>MDGGMWLMQQINGQVARMKSLGMQLEAADIYNPNGSSLKDAVVMFDGGCTGVLVSNQGLLLTNHHCGYDQIQKHSSVQHNYLKDGFWSYSLAEELVNPGLEVEIVDEITDVTAAVKKELERIKKPSGLEFLSPRYLSSLAPEIVGKKAASRPGYRYEIKAFYGGNRYYMFTKKVFRDVRLVAAPPSSIGKFGSDTDNWAWPRHTGDFSIFRLYADKNGNPAEYSKDNVPYRPKRWVKVNAQGVKEGDFALIMGYPGTTYKFFTADEVTEWSEIDNNIRIEMRGILQDVMLREMLADPKINIMYAAKYASSQNGYKRAQGANWAIRRRSLREIKLAQQQEVLAWAKQKGIATTEEAVRAISKAIEGRQDLRMRQRYLLEGILMGIEMSNAPAADSDIADHWDDPARREAGLQSIRKQFEAFFNKDYSPEVEKDQLAIALLTRYAERIPAEKQPISIREGIAEYGSAKAYVEMIFDKSIYASRERFEEFMKNPDRDRLLRDPMSRFAASVAYEHQKLAKEVAAFDAPLAAAQRSYVASVLDMKGQPNLAPDANLTLRFTYGEIKGYQPRDVVTYGA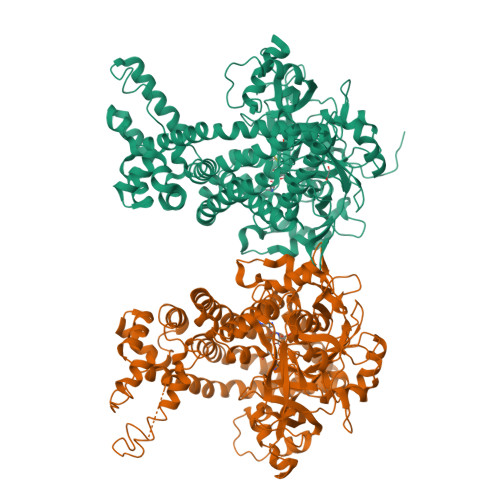KSTLEGVMEKEDPNNWEYVVDPKLKALYEAKNYGRYANSDGSMPVNFCATTHTTGGNAGSPVMNARGELIGLNFDRNWEGVGGDIEYLPNYQRSIILDIRYLLFIIDKFAGCQRLIDEIQPQFHHHHHH[2x]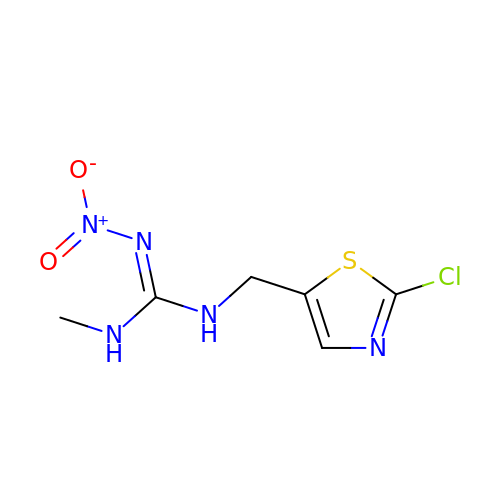1-[(2-chloro-1,3-thiazol-5-yl)methyl]-3-methyl-2-nitroguanidine | C6 H8 Cl N5 O2 S | PGOOBECODWQEAB-UHFFFAOYSA-N> STTLTRQDLNFGQVVADVLCEFLEVAVHLILYVREVYPVGIFQKRKKYNVPVQMSCHPELNQYIQDTLHCVKPLLEKNDVEKVVVVILDKEHRPVEK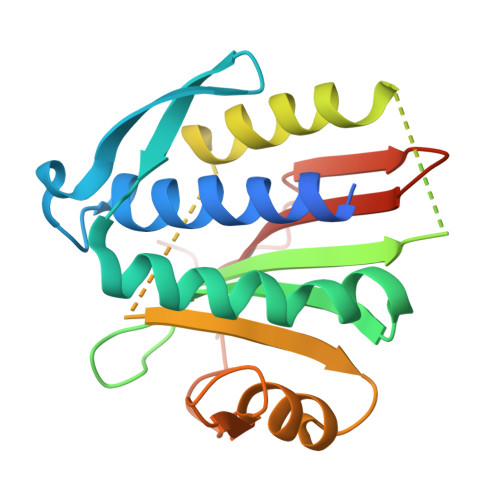FVFEITQPPLLSISSDSLLSHVEQLLRAFILKISVCDAVLDHNPPGCTFTVLVHTREAATRNMEKIQVIKDFPWILADEQDVHMHDPRLIPLKTMTSDILKMQLYVEERAHKGS>[2x]GSDFDFLKNLSLEELQMRLKAL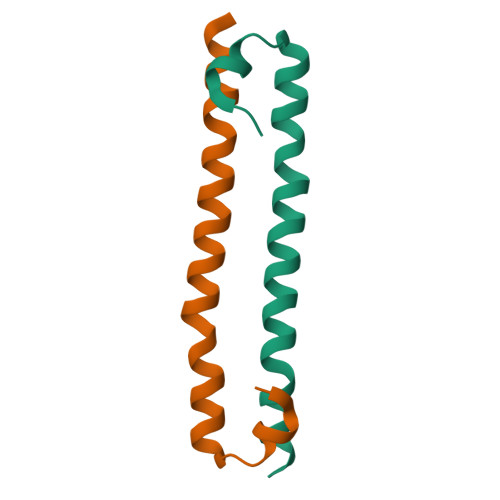DPMMEREIEELRQRYTAKRQPILDAMDAK>MHIERLAVDESVGRAMPPQRFIEALSDLGVPVEFAGEDEQFGPGDAVASFGHRDAFLDADWVHCIRAGYDEFPVGVYEEAGTYLTNSTGIHGTTVGETVAGYMLTFARRLHAYRDAQHDHAWDLPRYEEPFTLAGERVCVVGLGTLGRGVVDRAAALGMEVVGVRRSGDPVDNVSTVYTPDRLHEAIADARFVVLATPLTDETEGMVAAPEFETMREDASLVNVARGPVVVESDLVAALDSGDIAGAAL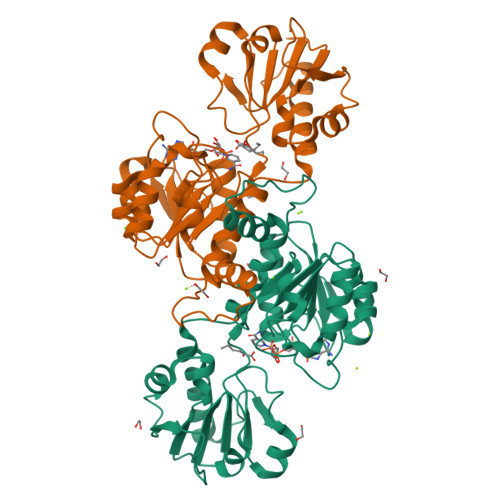DVFSEEPLPEDSPLWDFEDVLITPHVSAATSKYHEDVAALIRENIEKIATGDELTNRVV[2x]> MALPTP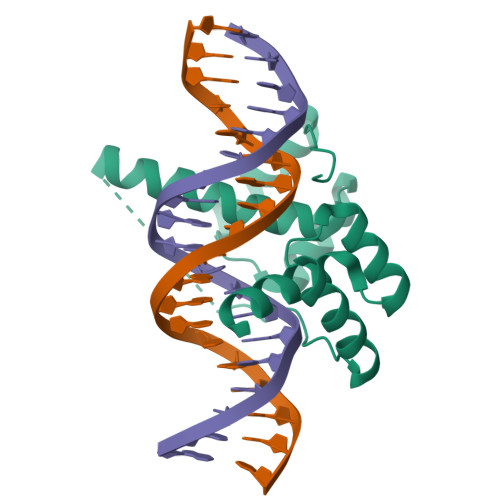SDSTLPAEARGRGRRRRLVWTPSQSEALRACFERNPYPGIATRERLAQAIGIPEPRVQIWFQNERSRQLRQHRRESRPWPGRRGPPEGRRKRTAVTGSQTALLLRAFEKDRFPGIAAREELARETGLPESRIQIWFQNRRARHPGQG>[2x]GMAHEAQKAIARNSLLIRSLPEQHVDALLSQAVWRSYDRGETLFLQEEKAQAIHVVIDGWVKLFRMTPTGSEAVVSVFTRGESFGEAVALRNTPY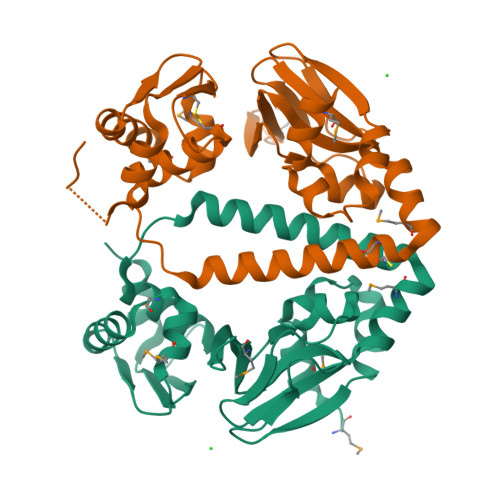PVSAEAVTPCEVMHIPSPVFVSLMRRDPEICISILATTFGHLHSLVAQLEQLKAQTGAQRVAEFLLELCDCDTGACEVTLPYDKMLIAGRLGMKPESLSRAFSRLKAAGVTVKRNHAEIEDIALLRDYAESDPADSWSKS>MAPKSSSSGSKKKSSASSNSADAKASKFKLPAEFITRPHPSKDHGKETCTAYIHPNVLSSLEINPGSFCTVGKIGENGILVIARAGDEEVHPVNVITLSTTIRSVGNLILGDRLELKKAQVQPPYATKVTVGSLQGYNILECMEEKVIQKLLDDSGVIMPGMIFQNLKTKAGDESIDVVITDASDDSLPDVSQLDLNMDDMYGGLDNLFYLSPPFIFRKGSTHITFSKETQANRKYNLPEPLSYAAVGGLDKEIESLKSAIEIPLHQPTLFSSFGVSPPRGILLHGPPGTGKTMLLRVVANTSNAHVLTINGPSIVSKYLGETEAALRDIFNEARKYQPSIIFIDQIDSIAPNRANDDSGEVESRVVATLLTLMDGMGAAGKVVVIAATNRPNSVDPALRRPGRFDQEVEIGIPDVDARFDILTKQFSRMSSDRHVLDSEAIKYIASKTHGYVGADLTALCRESVMKTIQRGLGTDANIDKFSLKVTLKDVESAMVDIRPSAMREIFLEMPKVYWSDIGGQEELKTKMKEMIQLPLEASETFARLGISAPKGVLLYGPPGCSKTLTAKALATESGINFLAVKGPEIFNKYVGESERAIREIFRKARSAAPSIIFFDQIDALSPDRDGSSTSAANHVLTSLLNEIDGVEELKGVVIVAATNRPDEIDAALLRPGRLDRHIYVGPPDVNARLEILKKCTKKFNTEESGVDLHELADRTEGYSGAEVVLLCQEAGLAAIMEDLDVAKVELRHFEKAFKGIARGITPEMLSYYEEFALRSGSSS[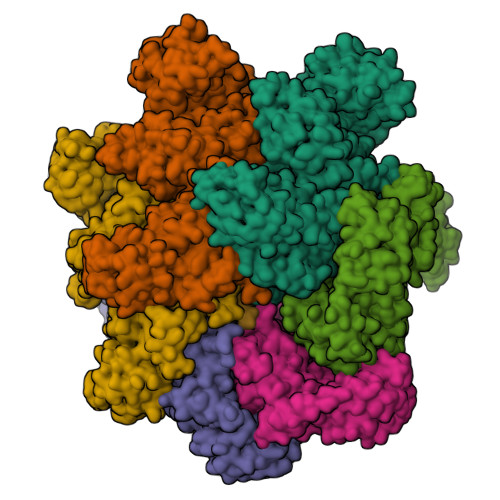6x]Herein, we report the identification of a distinct FPMO, CtdE, that stereoselectively catalyzes the 3S-spirooxindole formation in the 21R-citrinadin A biosynthesis. To gain insights into the mechanism of the stereoselective spirocyclization catalyzed by CtdE, the X-ray crystal structures of CtdE–FAD and CtdE–FAD-3 complexes were solved by molecular replacement, and refined to 2.1 and 1.9 Å resolution, respectively. CtdE comprises two domains, a three-layer ββα sandwich domain for FAD binding, and an internal substrate-binding domain featuring eight antiparallel β-sheets. We proposed that 3 may undergo a 2,3-β-face epoxidation as the first key step catalyzed by CtdE and followed by the regioselective opening of the epoxide ring that triggers the semipinacol rearrangement to form the 3S-spirooxindole 5.

The cofactor FAD was co-purified with CtdE without exogenous supplement during the protein purification and crystallization steps. In the CtdE–FAD complex, the FAD exists in the “out” conformation, in which the isoalloxazine moiety is away from the substrate-binding site, similar to that seen in PhqK24. Similar to the “mobile flavin” in para-hydroxybenzoate hydroxylase study, the “out” conformation could enable flavin reduction and substrate releasing, while the “in” conformation places flavin adjacent to the substrate and performs oxidation reactions. The CtdE–FAD complex features an open substrate loading channel, allowing the substrate to access the active site, whereas this substrate loading channel closed after substrate binding in the CtdE–FAD-3 structure. The FAD in its “out” and “in” conformations displays drastic changes in its interactions with surrounding residues. The residue R122 forms different hydrogen bonds with the hydroxy groups of flavin in the “out” and the “in” conformations, and is conserved in FPMOs PhzS (R106), HpxO (R103), and TropB (R124). Superimposing the CtdE–FAD complex onto the CtdE–FAD-3 revealed that the residues R122, R200, H229, L238, M253, and T333 move closer to 3 upon substrate binding. In addition, the polar residues D60 and Y249 move away from the substrate, which may provide a hydrophobic environment for substrate binding.

> MTKTPEAPVPRTMEKDHTQQINVIIVGLGIAGLTAAIECHRKGHKVIAFEKTPKMMHIGDIFSIGPNAESVIRQWKDGAISRALNEARCAIDEIKVFDETGKLQNVNTMEGYREGEGYVINRAEAVDIFFEYAQSLGIDIRFNSNVTEYWETPHNAGIIVDGLKIEADCVIATDGIHSKARNAICGAVVQPKKTGSAIYRSGYAMEELRGHSGAVWLTEGKEDVDQLYHFIGKDITVLVGTGRRGKDVYWGCMHKSLHDVSESWIQVSDVRRAIELISDWNVRDRLEPIMACTPQGKCFDHLVMTMDQLPSWVSPKHRMIVLGDAAHPFLPNTGQGANQAIEDGATVAICLELAGKNQVTKGVQVAERLRYQRVAKIQELGHRMLKTLQNADWDGEKDEDAPTMITRPAWIYSHDCQQYAYNEFQTVAQLVSERRDFHHHHHH3-[(Z)-(2,3-difluorophenyl)diazenyl]pyridine-2,6-diamine 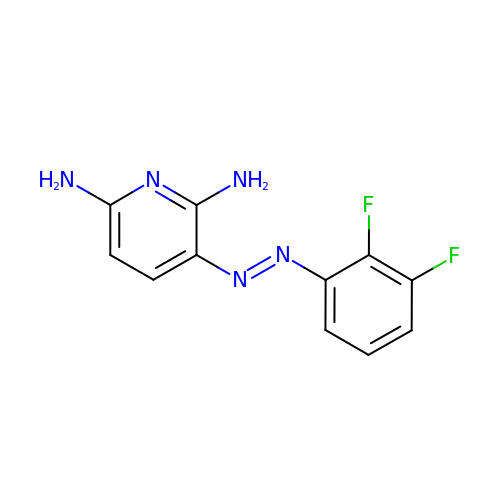| C11 H9 F2 N5 | KBEPGXDKUHLALK-UHFFFAOYSA-N>[6x]ATPHINAEMGDFADVVLMPGDPLRAKYIAETFLEDAREVNNVRGMLGFTGTYKGRKISVMGHGMGIPSCSIYTKELITDFGVKKIIRVGSCGAVLPHVKLRDVVIGMGACTDSKVNRIRFKD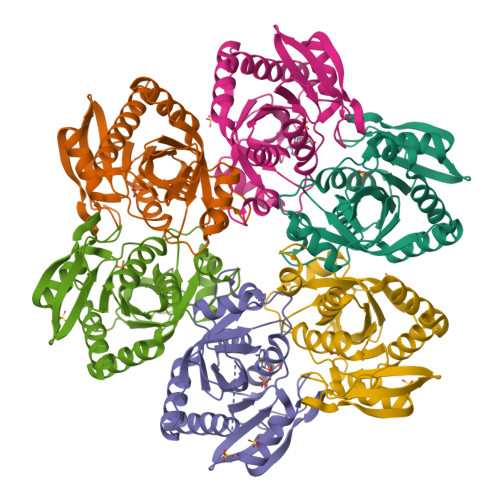HDFAAIADFDMVRNAVDAAKALGIDARVGNLFSADLFYSPDGEMFDVMEKYGILGVEMEAAGIYGVAAEFGAKALTICTVSAHIRTHEQTTAAEAQTTFNDMIKIALESVLLGDK>MVLYFIGLGLYDERDITVKGLEIAKKCDYVFAEFYTSLMAGTTLGRIQKMIGKEIRVLSREDVELNFENIVLPLA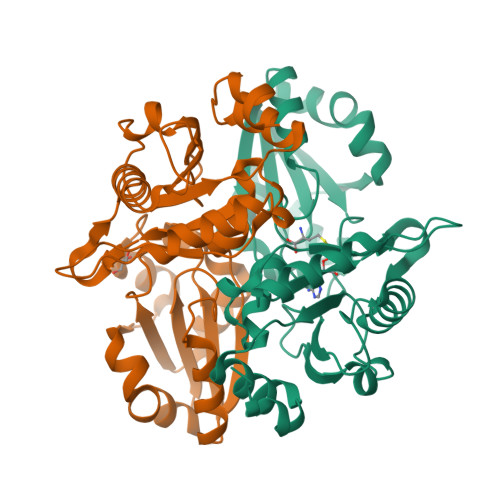KENDVAFLTPGDPLVATTHAELRIRAKRAGVESYVIHAPSIYSAVGITGLHIYKFGKSATVAYPEGNWFPTSYYDVIKENAERGLHTLLFLDIKAEKRMYMTANEAMELLLKVEDMKKGGVFTDDTLVVVLARAGSLNPTIRAGYVKDLIREDFGDPPHILIVPGKLHIVEAEYLVEIAGAPREILRVNV[2x]> GSTLQPLENSTRQEKLLYPKLNQLSNSINAAVAFLLEARNLEGWWQDFNFPQAASIGDEWVTAYVGTMLATLPYAHVHEALMQAWELLKIRDHRPTGEWGYNYILCGDADTTGWALQLAAAVGASDSERAQQARAALATHLQPNGGIATFAEESIRAYIKVPDLANVSFQGWCGAHTCVSAAVAALPEFRSRLHDYLRVTQTSQGNWEGYWWSDHEYTTALTAEALAAGGQAADQPSIEQAVAWGLKRLCPQGFVATSKHPNGSTFATAWCLRLLLLNTVDAEVKAARAAAIGWLLEQQRPNGSWVSSAYLRIPYPFDRNPNQFPHWRYYDEIEGDKAFEGSIIFDHN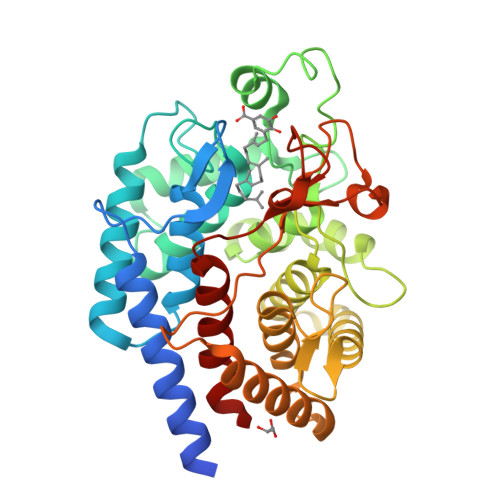SIFTTATVVNSLVKAAPML> STENLYFQSNADSVQNHTFEVENNTINGLELVEEQVHILYAMVLQTHAD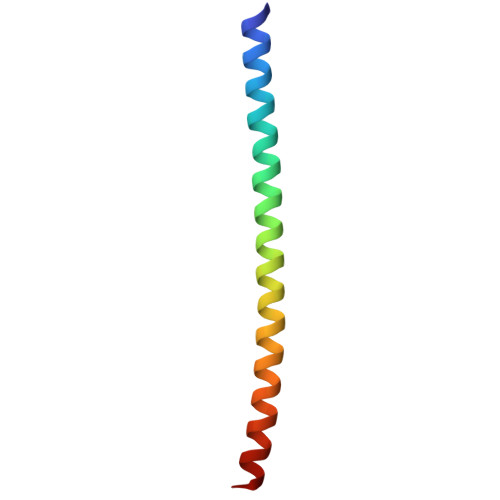VQLLKEQQ>[2x]MAHHHHHHDEVDMPGTKRFQHVIETPEPGKWELSGYEAAVPITEKSNPLTQDLDKADAENIVRLLGQCDAEIFQEEGQALSTYQRLYSESILTTMVQVAGKVQEVLKEPDGGLVVLSGGGTSGRMAFLMSVSFNQLMKGLGQKPLYTYLIAGGDRSVVASREGTEDSALHGIEELKKVAAGKKRVIVIGISVGLSAPFVAGQMDCCMNNTAVFLPVLVGFNPVSMARNDPIEDWSSTFRQVAERMQKMQEKQKAFVLNPAIGPEGLSGSSRMKGGSATKILLETLLLAAHKTVDQGIAASQRCLLEILRTFERAHQVTYSQSPKIATLMKSVSTSLEKKGHVYLVGWQTLGIIAIMDGVECIHTFGADFRDVRGFLIGDHSDMFNQKAELTNQGPQFTFSQEDFLTSILPSLTEIDTVVFIFTLDDNLTEVQTIVEQVKEKTNHIQALAHSTVGQTLPIPLK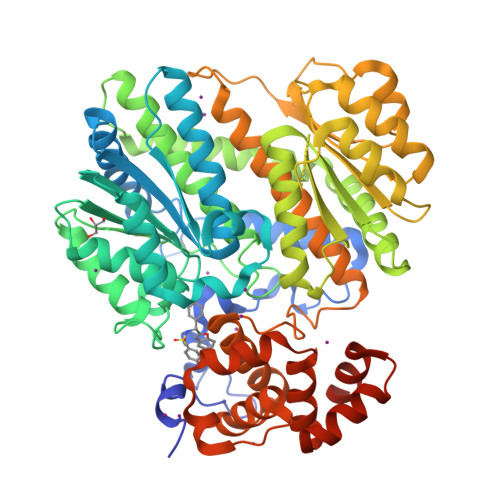KLFPSIISITWPLLFFEYEGNFIQKFQRELSTKWVLNTVSTGAHVLLGKILQNHMLDLRISNSKLFWRALAMLQRFSGQSKARCIESLLRAIHFPQPLSDDIRAAPISCHVQVAHEKEQVIPIALLSLLFRCSITEAQAHLAAAPSVCEAVRSALAGPGQKRTADPLEILEPDVQG(1~{R},3~{S},5~{Z})-4-methylidene-5-[(~{E})-3-[3-(6-methyl-6-oxidanyl-heptyl)phenyl]pent-2-enylidene]cyclohexane-1,3-diol 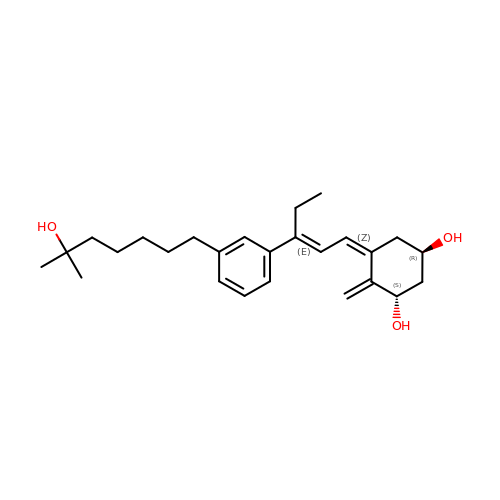| C26 H38 O3 | BQVXPWDQMUNMLU-FIKMVKLPSA-N>HHHHHHSSGLEVLFQGPMSDNTLSQKENMYPEINIKAMNQAVNTIWLLAQRQTSGIEIINDKVKRISLYSREFDEMMRDSLAQLAPVLKQLTSDAAFQTIAQIDEALADPSLSKDDREALTLERNNLIQNLSKHIDNVIVSFTGRTSKLTNKISDISDMVIAERLQDLVTQTESQKTELQSDIDPKTEKRNKLDADREKIIESQDVIRQNNIADMFKDFIPSAKDIDGLDFTQPKKEAIKQAIKQGAEIARKILGKVSEGLKYIDLADARMKLSDQIDQLITETDELKAKIREVELRLSGLKDVMQIDTERT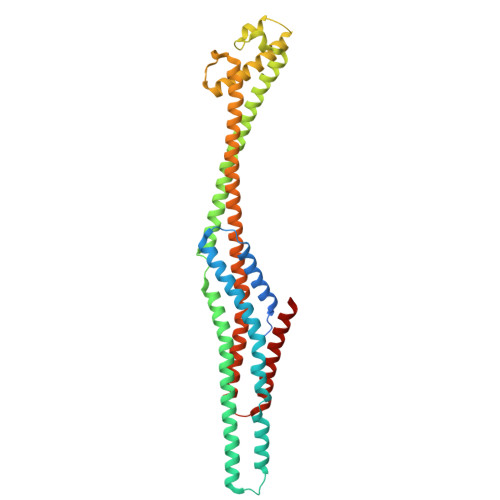TLLTEAVKIEQVWISFAEQLHKLSNDEINQQDLSNLINGQLDFLNNLTLQYNKLK[4x]> ATPSMMPQWSYMHISGQDASEYLSPGLVQFARATETYFSL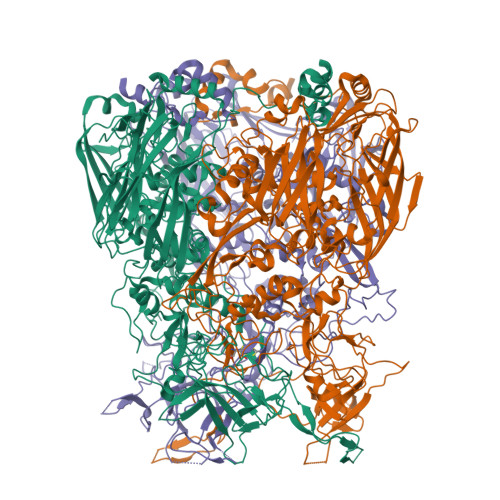NNKFRNPTVAPTHDVTTDRSQRLTLRFIPVDREDTAYSYKARFTLAVGDNRVLDMASTYFDIRGVLDRGPTFKPYSGTAYNALAPKGAPNPCEWDEAATALEINLEEEDDDNEDEVDEQAEQQKTHVFGQAPYSGINITKEGIQIGVEGQTPKYADKTFQPEPQIGESQWYETEINHAAGRVLKKTTPMKPCYGSYAKPTNENGGQGILVKQQNGKLESQVEMQFFSTTEATAGNGDNLTPKVVLYSEDVDIETPDTHISYMPTIKEGNSRELMGQQSMPNRPNYIAFRDNFIGLMYYNSTGNMGVLAGQASQLNAVVDLQDRNTELSYQLLLDSIGDRTRYFSMWNQAVDSYDPDVRIIENHGTEDELPNYCFPLGGVINTETLTKVKPKTGQENGWEKDATEFSDKNEIRVGNNFAMEINLNANLWRNFLYSNIALYLPDKLKYSPSNVKISDNPNTYDYMNKRVVAPGLVDCYINLGARWSLDYMDNVNPFNHHRNAGLRYRSMLLGNGRYVPFHIQVPQKFFAIKNLLLLPGSYTYEWNFRKDVNMVLQSSLGNDLRVDGASIKFDSICLYATFFPMAHNTASTLEAMLRNDTNDQSFNDYLSAANMLYPIPANATNVPISIPSRNWAAFRGWAFTRLKTKETPSLGSGYDPYYTYSGSIPYLDGTFYLNHTFKKVAITFDSSVSWPGNDRLLTPNEFEIKRSVDGEGYNVAQCNMTKDWFLVQMLANYNIGYQGFYIPESYKDRMYSFFRNFQPMSRQVVDDTKYKDYQQVGILHQHNNSGFVGYLAPTMREGQAYPANFPYPLIGKTAVDSITQKKFLCDRTLWRIPFSSNFMSMGALTDLGQNLLYANSAHALDMTFEVDPMDEPTLLYVLFEVFDVVRVHRPHRGVIETVYLRTPFSAGNATT> GMRQGAGLGYRRDLAEGFLQLRNNDRIQFMEIAPENWIKMGGFARYQFDKVAEKIPILIHGLSLSLGGQAPLDKELLSSIKAMIKQYNTPFFSDHLSFCECDGHLYDLLPMPFTDEAVKHTAARIREVQDFLEIQISVENTSYYLHSETSTMNEVEFLNAIVQEANCGIHLDVNNIYVNAVNHGLLDPHVFIDNVDLKRVNYIHIAGHDDEHAATEVQIQTSESFNKIKGDLRHLPPLLVDTHGENVKGTVWDLLEYTYARLSHMPPTLLERDFNFPPFEKLCKE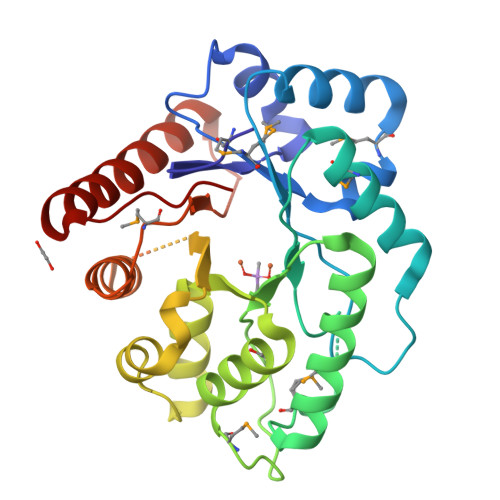VDIIHQLQQKYVKKRGLSWLKI3-nitrophenyl 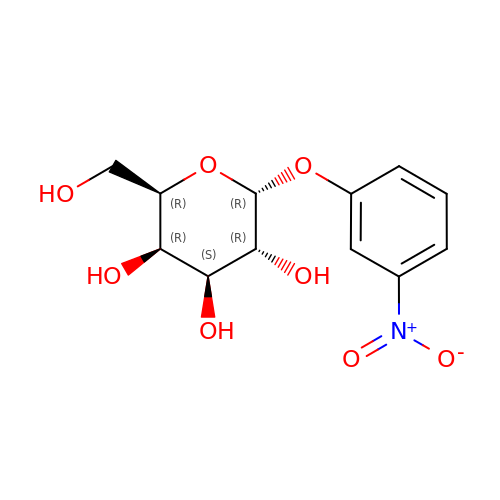alpha-D-galactopyranoside | C12 H15 N O8 | VCCMGHVCRFMITI-IIRVCBMXSA-N>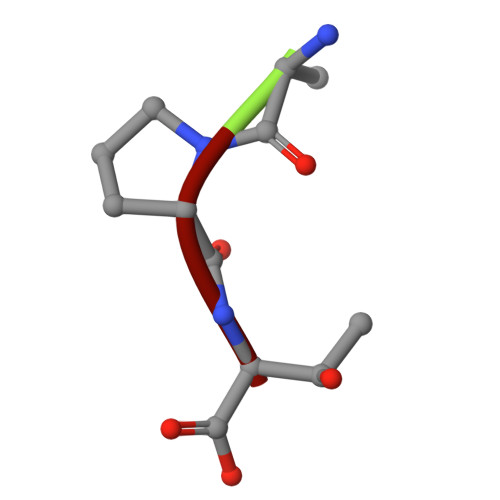 APT>MEKEHNPYNSETNLETNLENTNIKSTGPSADDLKSRFKEGSIPLQTDYADLIDIADIGRRAVGKAPDQTNNPNSALELDDNSGLKIKINSTGGLKADQDGLSVKLKDKSLLADPNGLAVNAGRGVKINNDQLEVDGYHGIEIVNEGVKVKASNGINVNSDGVSVKAGNGISVSGKGVEVKAKDKGSISVDSDGIAVKYWDGGGIVATDNSGLYLKLEGGNTNNGWSGVSGLSLSKNGVKVKAGNGITVDSSGVSIDPKTVLPKGMIVMFSGSSAPTGWAFCDGNHGTPDLRSRFVMCSETISETGKSSNKASGSGNGKNYSRNTTSTTVSVSVTVKNTTLTESQIPYHYHIGGMGYWTNKGMKYGTEYYSEYASYIRNDLDSVMQSANGARYAYTSPSGGGQGHNHPATASSPSHDHSVNVIPPYYLLAFIMKL[3x];>[3x]MNNQDALFPIVKDDIAFETLLTQAKTVIEQQSGQLWSNTEENDPGITLLEACCYGASDLAYRHSLPLRDLLTPEKQEQTLGDGIFPQEFGPQQMLTCGPITAEDYRRALLDLHSSDTDNETSEDYFFFNDVRLICEPESERYKYWYNKESREYSFIQEQEQEQEQLQLTLRGNYWLYLLPNRETEDDKTLTQKRLNDFLKDNRNLGESVSKIIWLQPVDFLLQLDIELDDDVSDLADIFAQVYMTTEQMVLTSPLRYSTQAMIEQGYSNEEIFEGPYLHHGWIPELSAAKDYTKPTELKLSHLANRLLAIPGVQNITRLALGKHDENISPLADDSWSWTIAQGYYPRLWGNDPLDLISSSASPLTITAKGGVKITVSKQDIENKIIAEPLIETQPELLNWGKHRKVLDYYPVSNKLPACYGLQTYAETQQQVHLHQFMLPFEQMLANGCAELALLPKLLAFKQRGNTVYGTQWPFKANTVGQQVHQEIMPDLIKQLNNDSQINSDDGIHSQNYTKELSILNYLLEYFGTHRAARPLTLDSLDFLSTQRGYLAQQPELTYQRNNIRIDKVSALQKRIAARLGLGGKCFEETSKLDELPFYLIEHRQLLPVKPDTKFDKEQKPDKLKIKSVPNSKNQQLIITQNGTTGQLLYGQVINLIIKEKEN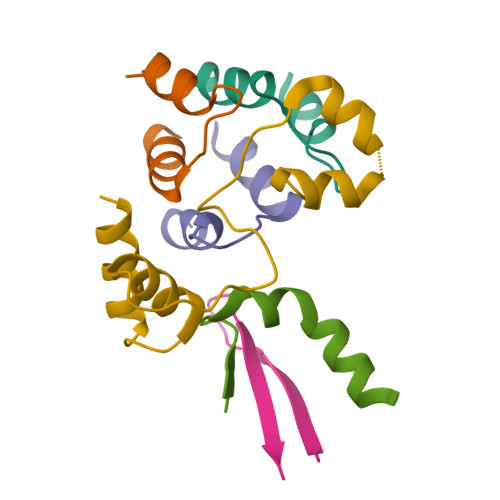QDIRVKFILRGQMITDITGESFILDTRNSTALARSLIDVQNAYNDGNLYWCNSPVWMEDMDYQLVYASEIYQTGTENERWITSSPQSPFPAMIEENDEITLKYVITPSGPKKSDHELKANVIKFDRIQGKILIKLTQDSQDNFPLAADAWRYRWYFSSEKYALADRFSFVVSMVINSQLVKNDDVDPYKLESWAKTEILAEFPAHLSMIIHWLSPEDFKDFVSTYQRWQNNGAPLGDEAYHVLETLTLGRLPSAATGIGNMRIATAQQRIGVVGESGKEWNTEVIISNQLVYVPYTGENLNKR> MKKQNDIPQPIRGDKGATVKIPRNIERDRQNPDMLVPPETDHGTVSNMKFSFSDTHNRLEKGGYAREVTVRELPISENLASVNMRLKPGAIRELHWHKEAEWAYMIYGSARVTIVDEKGRSFIDDVGEGDLWYFPSGLPHSIQALEEGAEFLLVFDDGSFSNSTFQLTDWLAHTPKEVIAANFGVTKEEISNLPGKEKYIFENQLPGSLKDDIVEGPNGEVPYPFTYRLLEQEPIESEGGKVYIADSTNFKVSKTIASALVTVEPGAMRELHWHPNTHEWQYYISGKARMTVFASDGHARTFNYQAGDVGYVPFAMGHYVENIGDEPLVFLEIFKDDHYADVSLNQWLAMLPETF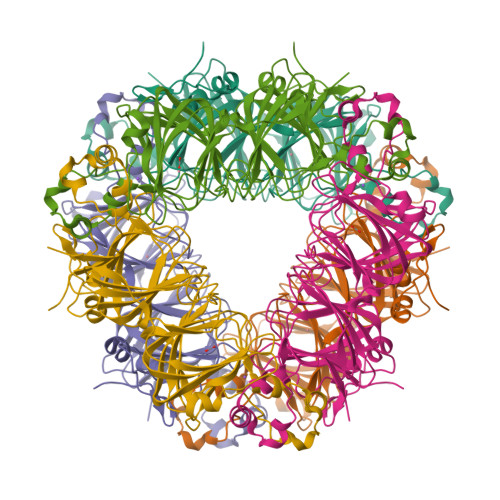VQAHLDLGKDFTDVLSKEKHPVVKKKCSKHHHHHH>MAEQTEQTTTPFVLPGLNYVHSGFPAPG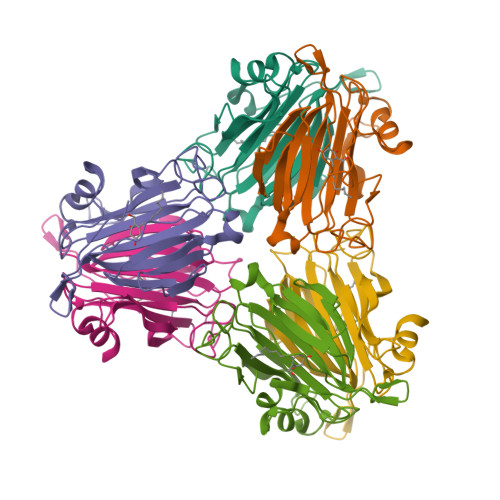LRQINRHITGHDDNGKSVFLSTDHGDHHRIMGEKQAVANILYSTQETPVQLNGNVDIDKAAKEEPPLHYHNGSIVRMIDFAPAVESPLHRAVSIDYGIVVEGVFKLVLDSGEERIMRQGDVSVQRATAHKWINITDNGTAPGRMMWILLDCHDVVVNGQVMEGYLGDLEKEYVGRGASK[12x]> QAGLNSRALWQFNGMIKCKIPSSEPLLDFNNYGCYCGLGGSGTPVDDLDRCCQTHDNCYKQAKKLDSCKVLVDNPYTNNYSYSCSNNEITCSSENNACEAFICNCDRNAAICFSKVPYNKEH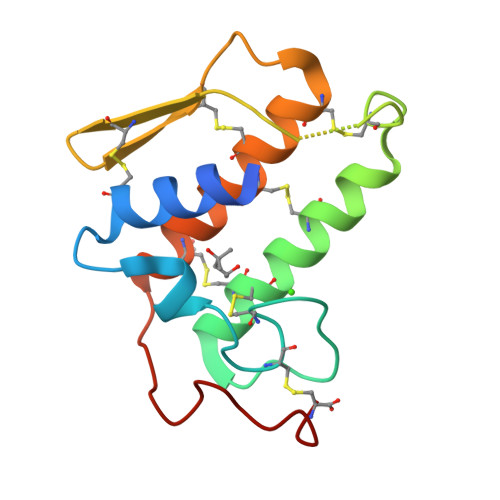KNLDKKNC(3-ENDO)-8-METHYL-8-AZABICYCLO[3.2.1]OCT-3-YL 1H-PYRROLO[2,3-B]PYRIDINE-3-CARBOXYLATE 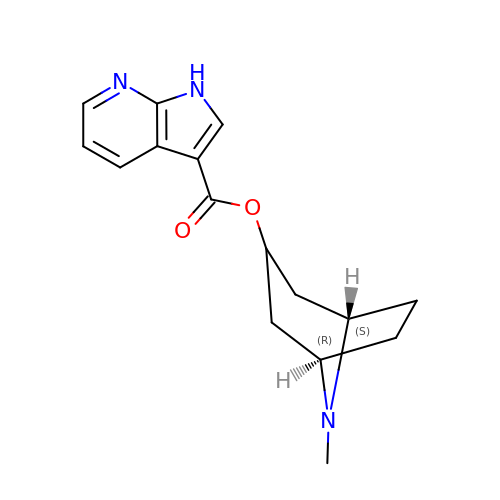| C16 H19 N3 O2 | WQGFCATXRXQKNB-GDNZZTSVSA-N>GIPGMLPWPKVDFSKFGEIEEVELGRIQKISGANLSRNWVMIPHVTHFDKTDITELEAFRKQQNEEAAKRKLDVKITPVVFIMKAVAAALEQMPRFNSSLSEDGQRLTLKKYINIGVAVDTPNGLVVPVFKDVNKKGIIELSRELMTISKKARDGKLTAGEMQGGCFTISSIGGLGTTHFAPIVNAPEVAILGVSKSAM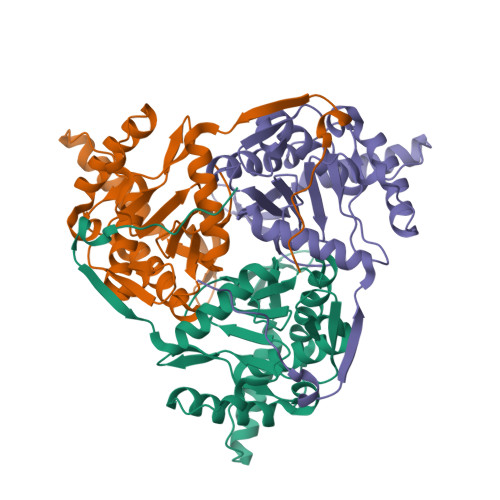EPVWNGKEFVPRLMLPISLSFDHRVIDGADGARFITIINNTLSDIRRL[4x]>MATDQMDISGPPPKKQHVDTESQIPKMYEMIRDQMRTLASTHKIPLNIDHNCEVIGSIIMAACTNNRDLRPVDKYWFLMGPAGAEVMTEVEIDIQPQLQWAKGAVHDPKYKGQWYPFLALLQISNKTKDTILWQKYPVTQELEISNSLEIYANGHGIKDRLKNSRPRSVGPLVHLLHLKRLQENPPKSPAVNGIRKSIVGHLKRQCIGETQKAMINQFEMGRWESLSTFAASLLAIKPRIENHFVLTYPLIANCEDFAGATLSDEWVFKAMEKISNKKTLRVCGPDEKWISFMNQIYIHS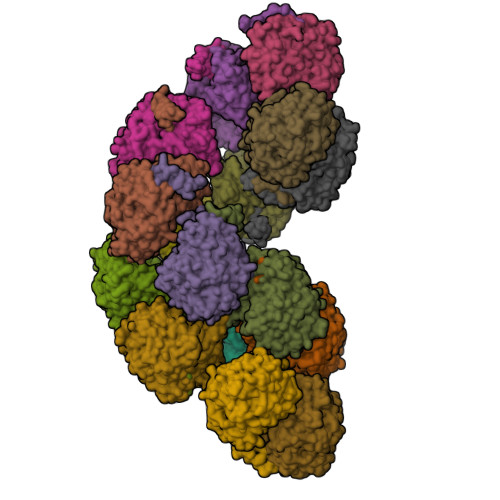VFQTTGEDLGVLEWVFGGRFCQRKEFGRYCKKSQTKVIGLFTFQYEYWSKPLKSAPRSIEGSKRGQISCRPSFKGKRPSYNNFTSIDALQSASGSQTVSFYDQVREECQKYMDLKVEGTTCFYRKGGHVEVEFPGSAHCNTYLFG[16x]>[2x]HHHHHHFNLPPGNYKKPKLLYCSNGGHFLRILPDGTVDGTRDRSDQHIQLQLSAESVGEVYIKSTET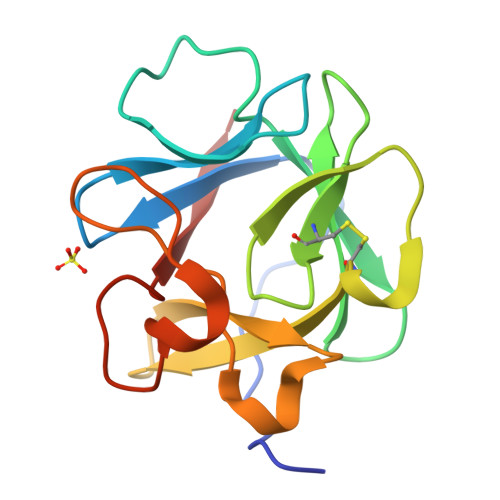GQYLCMDTDGLLYGSQTPNEECLFLERLEENHYNTYISKKHAEKNWFVGLKKNGSCKRGPRTHYGQKAILFLPLPVSSD>MSLSQVKHIILVLSGKGGVGKSSVTTQLALSLSQAGYSVGVLDVDLTGPSIPRMFAVEDAKVKQGSGGWLPVVVHEANPSTGIGSLRVMSLGFLLPRRGDAVIWRGPKKTAMVRQFMSDVLWDELDFLLVDTPPGTSDEHISLAETLLQEARPGQLSGAIVVTTPQAVATADVRKELNFCKKTGIRVLGVVENMSGFVCPNCSECTNIFSSGGGEIMANDFNVRFLGRVPIDPQFLVLIETGKRPRYPEGTKVNSQDLSFQHLEQVDNADNPETPNSSLLVDKY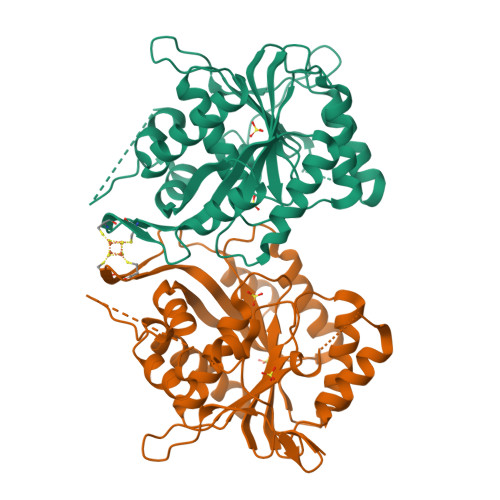RDCSLAPIFRAITADVVVAVEQASGS[2x]> MAPARENVSLFFKLYCLTVMTLVAAAYTVALRYTRTTAEELYFSTTAVCITEVIKLLISVGLLAKET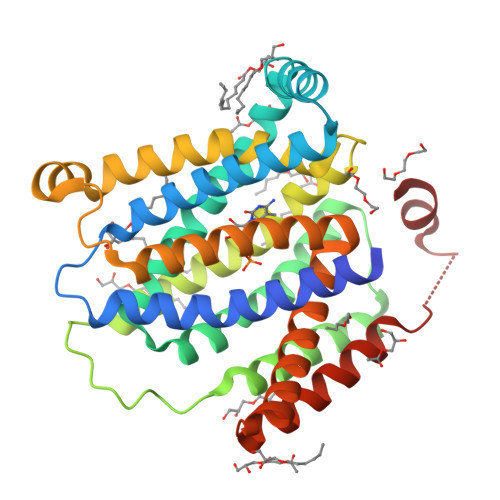GSLGRFKASLSENVLGSPKELAKLSVPSLVYAVQNNMAFLALSNLDAAVYQVTYQLKIPCTALCTVLMLNRTLSKLQWISVFMLCGGVTLVQWKPAQATKVVVAQNPLLGFGAIAIAVLCSGFAGVYFEKVLKSSDTSLWVRNIQMYLSGIVVTLAGTYLSDGAEIQEKGFFYGYTYYVWFVIFLASVGGLYTSVVVKYTDNIMKGFSAAAAIVLSTIASVLLFGLQITLSFALGALLVCVSIYLYGLPRQDTTSNSLEVLFQ> MIHLIALRLTRGMDLKQQIVQLVQQHRIHAGSIASCVGCLSTLHIRLADSVSTLQVSAPFEILSLSGTLTYQHCHLHIAVADAQGRVWGGHLLEGNLINTTAELMIHHYPQHHFTREFDPNTGYSELVVSAAA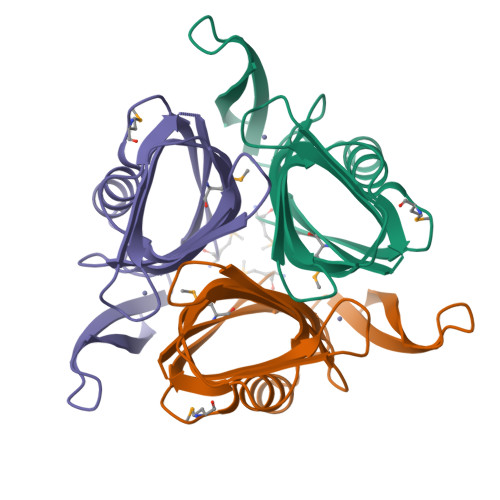LEHHHHHHH(5R,9S,12S,15S,18S,21S)-21-benzyl-12,18-bis(carboxymethyl)-15-cyclohexyl-1-(9H-fluoren-9-yl)-4-methyl-9-(2-methylpropyl)-3,6,10,13,16,19-hexaoxo-5-phenyl-2-oxa-4,8,11,14,17,20-hexaazadocosan-22-oic 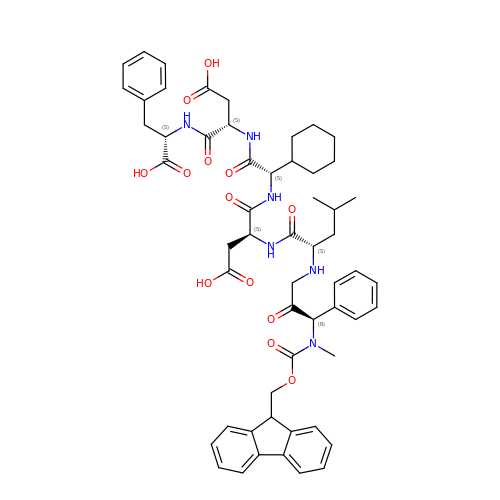acid | C56 H66 N6 O13 | VHDDRUTXAIHKQU-NXKHAHLZSA-N>LVPRGSEDKWRNAFDHMLMEEFEEKMDQIEHGLLMLSEQYKELEKTKSKELKEQILRELTIAENYLRGALKFMQQEAKRTDLNMFERYNFETAVSTIEILVKDLAELAKKVKAVKSDDGSHHHHH[2x];>[2x]MLPDEEKLKLLDTLLTMVEWVKELLEESVEKNSRMRHIRAVMWAEYMLEIARSLEDEKILEIAEKLEKALPEKSKMFTKEEYEKLMEVLEELEEVLEEKKEE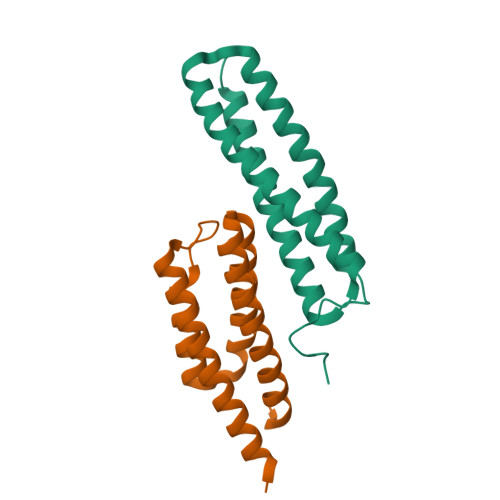VEERIEGSHHHHH>MGSSHHHHHHSQDPSNDNQDDDGRIHDKMKRRLAQNREAARKSRLRKKAYVQQLEESRLKLSQLEQELEKVKQQGHLGPSGSINTGIASFEMEYSHWLQEQSRRVSELRTALQSHISDIELKMLVESCLNHYANLFQMKSDAAKADVFYLISGMWRTSTERFFQWIGGFRPSELLNVVMPYLQPLTDQQILEVRNLQQSSQQAEDALSQGIDKLQQSLAESIVIDAVIESTHYPTHMAAAIENLQALEGFVNQADHLRQQTLQQMAKILTTRQSARGLLALGEYLHRLRALSSLWAARPQ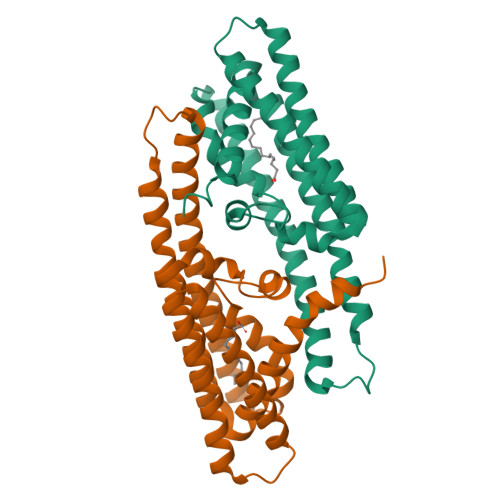EPT[2x]>[6x]SIIQVFFIAGRTDEQKERLIGALTDAAVKTIGIDRSDVRVILKDIPNTEYGIAGK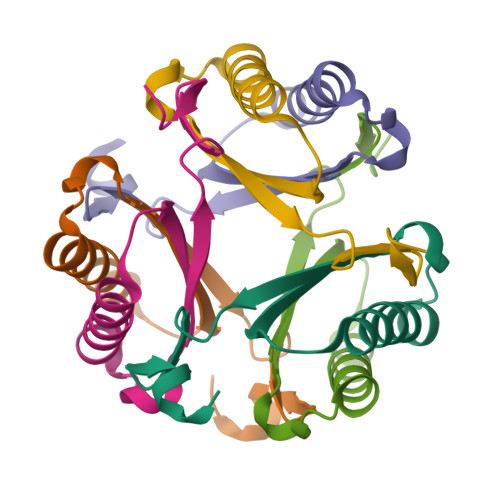TAKSLGRGTGRSPAGS;>[6x]PNIEMFVVEGLSDQQKEKLIDALTAATVEAIDAPADSIRVWLSEIPAKQFGIAGKSVAAIEAARKNK(3~{S})-19-chloranyl-~{N}-(1-cyanocyclopropyl)-8-methoxy-5-oxidanylidene-12,17-dioxa-4-azatricyclo[16.2.2.0^{6,11}]docosa-1(20),6(11),7,9,18,21-hexaene-3-carboxamide | C25 H26 Cl N3 O5 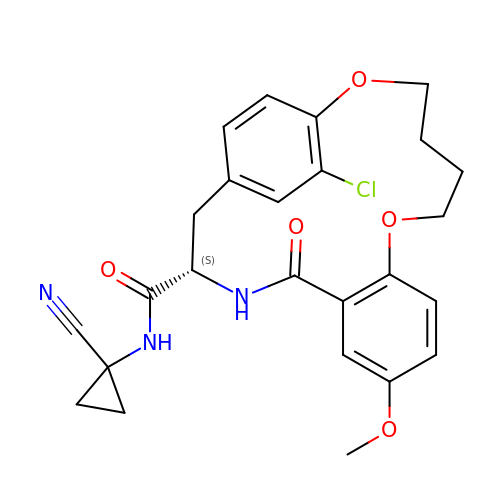| QAEMDWMOUWWGNG-FQEVSTJZSA-N5,10-METHENYL-6,7,8-TRIHYDROFOLIC ACID | 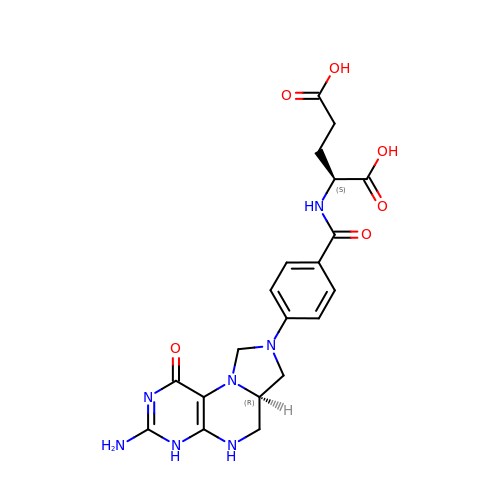C20 H23 N7 O6 | QYNUQALWYRSVHF-OLZOCXBDSA-N> AMDSPGVFFDSDKGKTHSSGKVLYNARIIPYRGSWLDFEFDPKDNLFVRIDRRRKLPATIILRALNYTTEQILDLFFEKVIFEIRDNKLQMELVPERLRGETASFDIEANGKVYVEKGRRITARHIRQLEKDDVKLIEVPVEYIAGKVVAKDYIDESTGELICAANMELSLDLLAKLSQSGHKRIETLFTNDLDHGPYISETLRVDPTNDRLSALVEIYRMMRPGEPPTREAAESLFENLFFSEDRYDLSAVGRMKFNRSLLREEIEGSGILSKDDIIDVMKKLIDIRNGKGEVD;> AMDVS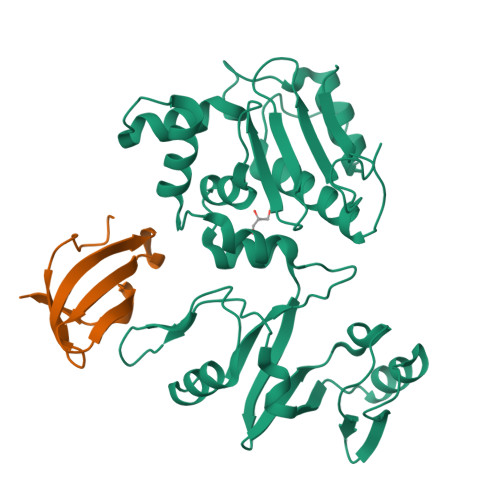HQRMGTPMVENDSGYKLGQRVRHAKFGEGTIVNMEGSGEHSRLQVAFQGQGIKWLVAAYARLESV>[7x]SMHSQPQTVTVDQQEILNRADEVEAP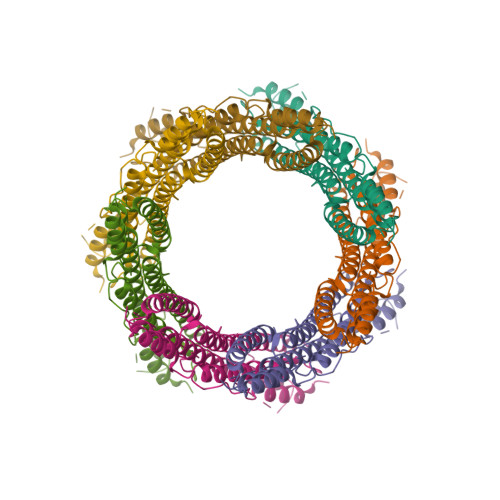MATPPTDVPQAPSGLTAANNAAEQLAVSADNVRLYLQAGERERQRLATSLRNAAAAYGEVEDESATALDNDGNGEVDAQSAGGAGAGQTESLEETPKVAAAGESDFTDLKTAATKLESGDQGTSMVNFADGWNNFNLSLQRDIKRFRIFENWEGDAATACEASMDQQKEWILHMAKLSASLAKQANFMAQLQLWARRGHPTLADIVELERLAKDPDYQEQAIKLYAEYQETSEKVLSEYNTKADLEPVNPPKPPAAIKIDPP>[5x]MYMSKYVPV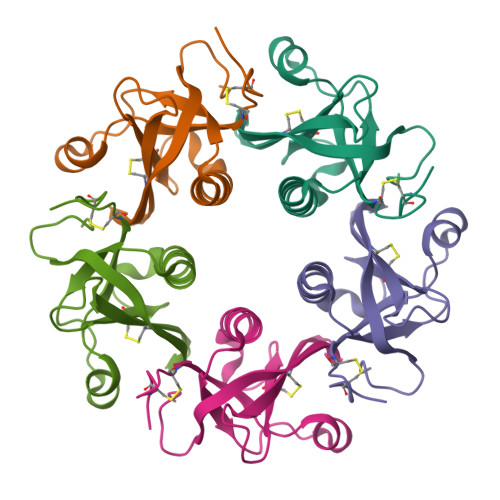YTLLILIYSFNASAEWTGDNTNAYYSDEVISELHVGQIDTSPYFCIKTVKANGSGIPVVACAVSKQSIWAPSFKELLDQARYFYSTGQSVRIHVQKNIWTYPLFVNTFSANALVGLSSCSATQCFGPKLEHHHHHH>AERTMFYGKGDVYVFRTYANPLK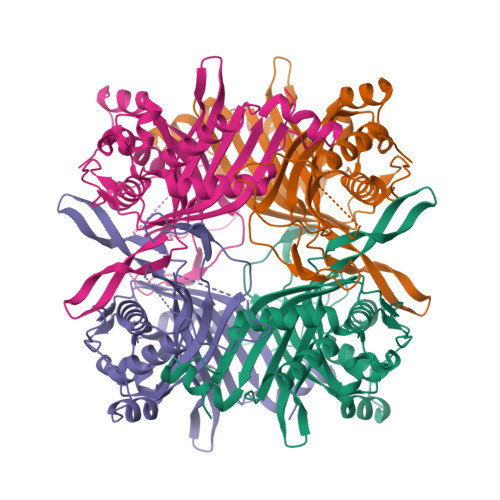GLKQIPESNFTEKHNTIFGMNAKVALKGEQLLTSFTEGDNSLVVATDSMKNFIQRHAASYEGATLEGFLQYVCEAFLAKYSHLDAVRLEAKEYAFDDIQVGTDKGVVTSDLVFRKSRNEYVTATVEVARTASGTEVVEQASGIADIQLIKVSGSSFYGYIIDEYTTLAEATDRPLYIFLNIGWAYENQDDAKGDNPANYVAAEQVRDIAASVFHTLDNKSIQHLIYHIGLTILDRFPQLTEVNFGTNNRTWDTVVEGTDGFKGAVFTEPRPPFGFQGFSVHQEDLAREKASANSEYVAL[4x]>HHHHMRIEVKLLPLKDNPILPFNYNYEVYSQILEKVNSIEPTIAKLLSSPHGFWTFSRIIVRKRKILPDKGIEILSDDVSLYISSSNEDIIRAIAEAVEKSPEFKIGELSFLVGDIKAIKVKELGKENVFSTLSPIVVRTVKFEGNKLRHWDLYPHDEL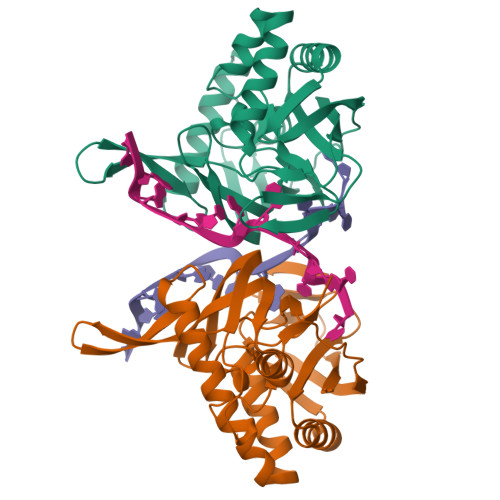FMDRLRKVMILRYSEVMGETPKDRDFTIEVLKFKPTRLMVGSSYIRGSLMVFRYAGSEEIARFGYENGFGEKTGLGFGMVKLIE[2x]>[4x]GAMGGPQEYTLIKLKIHLIPEFLGSIVKGREVFVVCATLRPETMYGQTNCWILPDGEYDLVLAFDQVIPYDAKTSDGVLCKIFDKYEDTMKECNTVYICSERSAYNMAYQGIVPLIHGREQGVSDKLLPRIVSLGKVYGEQLIGTPLSAPMTPYSLIFILPMFSISMEKGTGIVTSVPSDSPDDYAALRDIKTKPLLREKYSIKD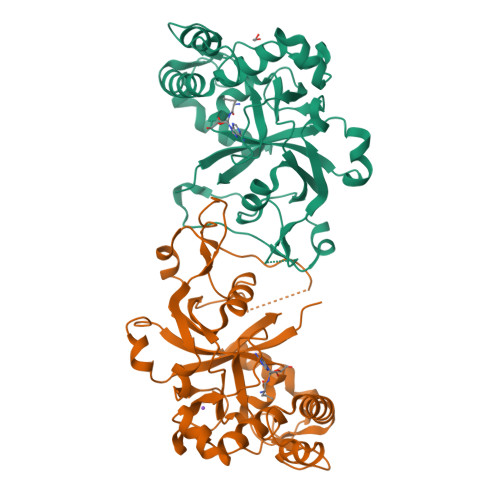EWILDPLEIIEVPGFGFMTAELLCNQYKIQSQNDSAKLKQAKEEIYKKEFYEGILIRGKYSGMKICDAKELIRESLIKDGYALIYLE SALICYLALDEHYDE | C7 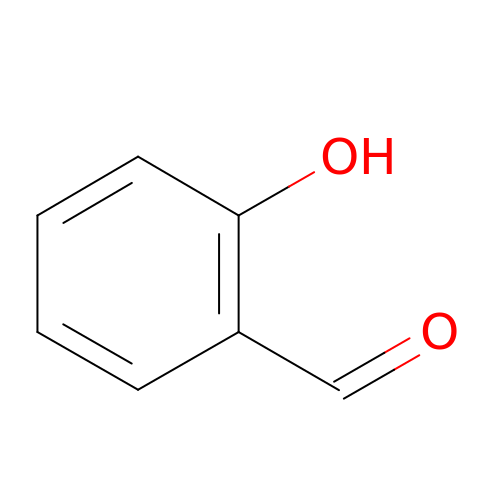H6 O2 | SMQUZDBALVYZAC-UHFFFAOYSA-N> MGSSHHHHHHSSGLMDSLLGCGVSAAAREPVPRYLTSQPRVSEVAMQSAPLEQPAKRPRCDGSPRTPPSTPPATANLSADDDFQNTDLRTWEPEDVCSFLENRGFREKKVLDIFRDNKIAGSFLPFLDEDRLEDLGVSSLEERKKMIECIQQLSQSRIDLMKVFNDPIHGHIEFHPLLIRIIDTPQFQRLRYIKQLGGGYYVFPGASHNRFEHSLGVGYLAGCLVRALAEKQPELQISERDILCVQIAGLCRNLGHGPFSHMFDGRFIPRARPEKKWKHEQGSIEMFEHLVNSNELKLVMKNYGLVPEEDITFIKEQIMGPPITPVKDSLWPYKGRPATKSFLYEIVSNKRNGIDVDKWDYFARDCHHLGIQNNFDYKRFIKFARICEVEYKVKEDKTYIRKVKHICSREKEVGNLYDMFHTRNCLHRRAYQHKISNLIDIMITDAFLKADPYVEITGTAGKKFRISTAIDDMEAFTKLTDNIFLEVLHSTDPQLSEAQSILRNIECRNLYKYLGETQPKREKIRKEEYERLPQEVAKAKPEKAPDVELKAEDFIVDVIN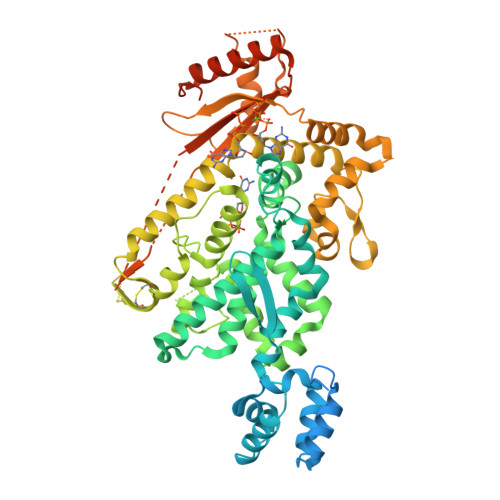VDYGMEDKNPIDRVHFYCKSNSKQAVRINKEQVSQLLPEKFAEQLIRVYCKKKDGKSLDAAGKHFVQWCALRDFTKPQDGDIIAPLITPLKWNNKTSSCLQEVSKVKTCLKF> MGSSHHHHHHSSGRENLYFQGMSTDFDRIYLNQSKFSGRFRIADSGL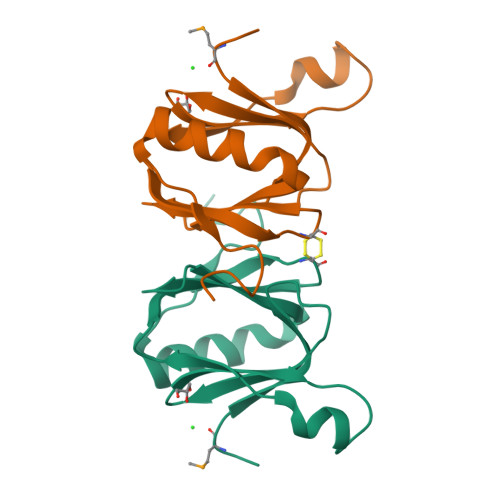GWKISTSGGSAANQARKPFLLPATELSTVQWSRGCRGYDLKINTKNQGVIQLDGFSQDDYNLIKNDFHRRFNIQVEQREHSLRGWNWGKTDLARNEMVFALNGKPTFEIPYARINNTNLTSKNEVGIEFNIQDEEYQPAGDEGS>[2x]MIHHVELTQ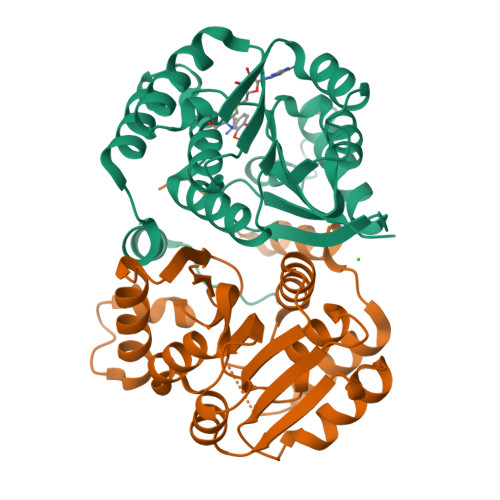SVLQYIRDSSVRDNDILRDLREETSKLPLRTMQIPPEQGQLLSLLVRLIGARKTLEVGVFTGYSTLCTALALPADGRVIACDLSEEWVSIARRYWQRAGVADRIEVRLGDAHHSLEALVGSEHRGTFDLAFIDADKESYDFYYEHALRLVRPGGLIILDNTLWSGKVADPSVVGDPETDSLRRINAKLLTDERVDLSMLPIADGLTLARKRKLAAALEHHHHHH> IPRSPVVTIMGHVDHGKTTLLDKLRKTQVAAMEAGGITQHIGAFLVSLPSGEKITFLDTPGHAAFSAMRARGTQVTDIVILVVAADDGVMKQTVESIQHAKDAHVPIVLAINKCDKAEADPEKVKKELLAYDVVCEDYGGDVQAVHVSAL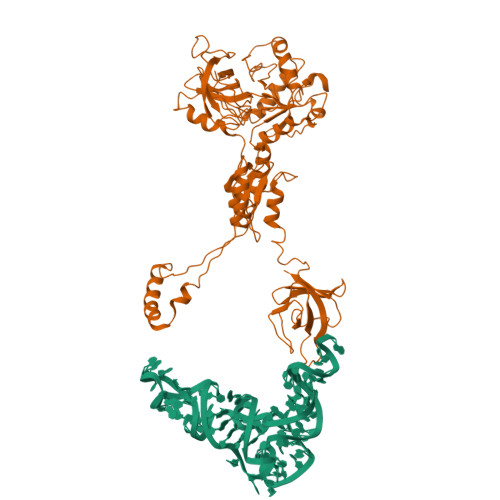TGENMMALAEATIALAEMLELKADPTGAVEGTVIESFTDKGRGPVTTAIIQRGTLRKGSILVAGKSWAKVRLMFDENGRAVNEAYPSMPVGIIGWRDLPSAGDEILEVESEPRAREVVDWRKYEQEQEKNKEDLKLIEEKRKEHQEAHRKDREKYGTVHWKERSYIKYREKRQQQPLKPKEKLERDSNVLPVIVKGDVDGSVEAILNVMDTYDASHECELDLVHFGVGDISENDVNLAETFHGVIYGFNVNAGNVIQQLAAKKGVKIKLHKIIYRLIEDLQEELSSRLPCIVEEHPIGEASILATFSITEGKKKVPVAGCRVQKGQIEKQKKFKLIRNGHVIWKGSLISLKHHKDDTSVVKTGMDCGLSLDEEKIEFKVGDAIICYE> MVLFTRCEKARKEKLAAGYKPLVDYLIDCDTPTFLERIEAIQEWDRSRDDLYVWIPILDRMDGLLLKVAEKYKYKQDPKKECEVKLVEMEAHDVDYCLKMLKFTRRLLLNTENRFVYSSGDVLMYLLNCPNFTIKLAVMRILAILGERFVIAREKIVAHNIFGDHNLRKKTLKLALSLSSSVMDEDGEHFSLVDLYFDKKKVPQKWRKLRFTHYTSNDFKKSSQQKNNINETQTSIKKVTMTTQELCEHSLQQIFDKGMALLPAESWFDFSIKASVAKAFSDDSGENIDLRNIIIETKLNAIAFVNTIFSPPQVSSKLFELDPYAFNSLTDLISLSETKIPKELRTDALFTLECISLKHVWCSDIIRNLGGNISHGLLFQILRYIAKTLREATDEIDEEYNVRFFYLISNLADVKPLHESLFAAGLIPTLLEIVSIRNCPYKRTLASATHLLETFIDNSETTTEFIENDGFTMLITSVANEIDFTLAHPETWQPPKYSVVYYSISFRELAYIRSLLKLVLKLLSTDSGDRIRNLIDSPILVSLKKILENKLVFGLTLITYTLDVVQKVINSEPTIYPVLVEAGLIPYVIDNFPKLIGPSAELLSLLPDVVSAICLNPEGLKQVKEKGLINNLFDFLLDADHARILTGGDRSTEYGTDIDELARHYPDLKANIVEALCNVIRKMPSTFRNEREFLFTSPKDQKYFFHRKNEEILTDKEEHEPAYWELLDKGTMLDTFTSVLFGMSLGNGSFSQVPQHLEARDFLAIIFMENPPYEYFTSVAISNVTEVLQYLDEKYEDYAFMDVMKVLNDQLENLNDFLNSPNDRSFFLERDGENSVRSCHSKLCRLAAILNIVTNVYIDLTTLSCKRIMQIYSYFDKRGFSLIKNLKLLFQKCALEEMYIRQHMPDSVITETMPLPIVDVSGDGPPLQIYIDDPKKGDQKGKITSVKTRNTLQMRTILYTLQSNTAILFRCFLRLSHSRNMDLEHK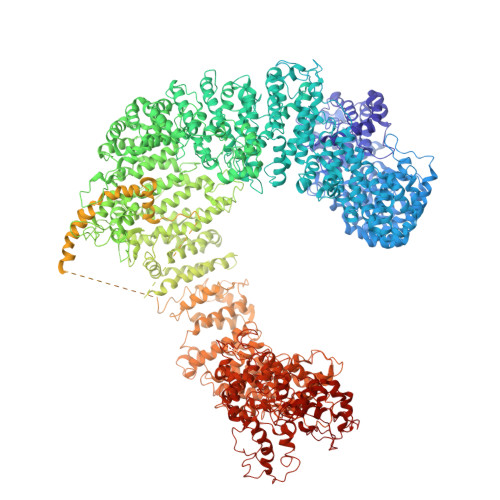DLTTEVHIFENVVENVIEMLKATELEGHLPYILVLLNFNTFVFTIPKASPNSTEILQTIPAYIFYQKGGYLLYLHIIRDLFTRMTKIKSGGGGGGSRHHHHHHHHHHHHDLSSLDNINYIDESNGILTLSCLINALTFYNKSMQTETMENVQSIGKYYVSIDDDYNIMKALTVPIKVMALAMILDLDKSDSLFKTQSRNVPYSVFKQLLSMLKNIFTNVNIYTKELYELHWDLIFPPIKKISLFEQVGIPGDVAANYLTDTGDDLPADNSIGLFSPEQWEKYKKLIGEDKSIYYPQPMQAQYYKGCSSKELDELRDTFFNDGLPSRIFTVLPFYPKLVNAFAKTLLQIFTKYDEPTEVFAGRILDRILETDLDDPATLSSLIHLFGIFLNEKYIYQKASHLMQRFIEYLEKSLKPEHVNTPWFSKALYVYEIILAKSELPHLEELSKDVLLRYPLLSMAKVFRIPDPMKQKLFDILIRVSDISNFYSALATSRILIFYSRDELYANNIARSGILSRLLKVIGSFQKLDKINFLESSFLLLTRRCFETTENVDALIRAEINRSFTARPLGGGDDAVRELTTILEEKAHVVMRSPSQFIDVLCETARFHEFDDQGALVDYSLKRFLGEKDKNTQASSTEKSDIYERTGIMHLLLSQLMAASEKDWLSEPANSSDLPENKKAQLDPSRNPVCAYMIFLLKLLVELVSSYNQCKFEFLTFSRRNTYAERPRPRTTAINFFLYRLLDKPVGTDHDKHEAKRREVIGMLARSVIIGFLATVQDDRTTKTDVKLADPHMNFIRKFAIEAIIKAIRNATSSSKLLESNHLKLDMWFRIITSMVYVQAPYLRQLLDSNKVEADQYQLCKLVIDLGLPSVITEAMASIDLNYPFSKKIFNVAVEALNTISSTRNNFSEHFKIEDHDEVEDEVDESDKEEIPDMFKNSALGMYDVEDIEEDDDDDTSLIGDDDAMAFVDSDNGFEVVFSDEDDDMGEEDADDARSDSEENELSSEMQSSTADGTDVDYEVDDADGLIINIDQPSGDDEEMADYDANISHSSHSENEDDASMDVIEVYDDELSSGYDVDLSDYDVDESDWDSGLSSLSISDEDSESSEDEPINSTRMGDSRRRWLIAEGVELTDDSQGESEEDDRGVFRGIEHIFSNENEPLFRVHDEMRHRNHHRSINRTHFHSAMSAPSLSLLNRGRRNQSNLINPLGPTGLEQVENDISDQVTVAGSGSRPRSHHLHFSEVLVSGSFFDEPVLDGIILKSTVSRWKDIFDMFYDSKTYANCIIPTVINRLYKVSLALQKDLENKREQEKLKNKNLLFNEAKVESHNSSDAISVEQDDIQESNVTHDDHEPVYVTIQGSEVDIGGTDIDPEFMNALPDDIRADVFAQHVRERRAEARLNSDHNVHSREIDSDFLEAIPEDIREGILDTEAEEQRMFGRIGSSADVIRADDDVSNNDEEVENGLDHGNSNDRNNADPEKKKPARIYFAPLIDRAGIASLMKSVFISKPYIQREIYHELFYRLCSSKQNRNDLMNTFLFILSEGIIDQHSLEKVYNIISSRAMGHAKTTTVRQLPSDCTPLTVANQTIEILQSLIDADSRLKYFLIAEHDNLIVNKANNKSRKEALPDKKLRWPLWHLFSLLDRKLITDESVLMDLLTRILQVCTKTLAVLSTSSNGKENLSKKFHLPSFDEDDLMKILSIIMLDSCTTRVFQQTLNIIYNLSKLQGCMSIFTKHLVSLAISIMSKLKSALDGLSREVGTITTGMEINSELLQKFTLPSSDQAKLLKILTTVDFLYTHKRKEEERNVKDLQSLYDKMNGGPVWSSLSECLSQFEKSQAINTSATILLPLIESLMVVCRRSDLSQNRNTAVKYEDAKLLDFSKTRVENLFFPFTDAHKKLLNQMIRSNPKLMSGPFALLVKNPKVLDFDNKRYFFNAKLKSDNQERPKLPITVRREQVFLDSYRALFFKTNDEIKNSKLEITFKGESGVDAGGVTREWYQVLSRQMFNPDYALFLPVPSDKTTFHPNRTSGINPEHLSFFKFIGMIIGKAIRDQCFLDCHFSREVYKNILGRPVSLKDMESLDPDYYKSLVWILENDITDIIEETFSVETDDYGEHKVINLIEGGKDIIVTEANKQDYVKKVVEYKLQTSVKEQMDNFLVGFYALISKDLITIFDEQELELLISGLPDIDVDDWKNNTTYVNYTATCKEVSYFWRAVRSFDAEERAKLLQFVTGTSKVPLNGFKELSGVNGVCKFSIHRDFGSSERLPSSHTCFNQLNLPPYESYETLRGSLLLAINEGHEGFGLA> MRSKRFEALAKRPVNQDGFVKEWIEEGFIAMESPNDPKPSIKIVNGAVTELDGKPVSDFDLIDHFIARYGINLNRAEEVMAMDSVKLANMLCDPNVKRSEIVPLTTAMTPAKIVEVVSHMNVVEMMMAMQKMRARRTPSQQAHVTNVKDNPVQIAADAAEGAWRGFDEQETTVAVARYAPFNAIALLVGSQVGRPGVLTQCSLEEATELKLGMLGHTCYAETISVYGTEPVFTDGDDTPWSKGFLASSYASRGLKMRFTSG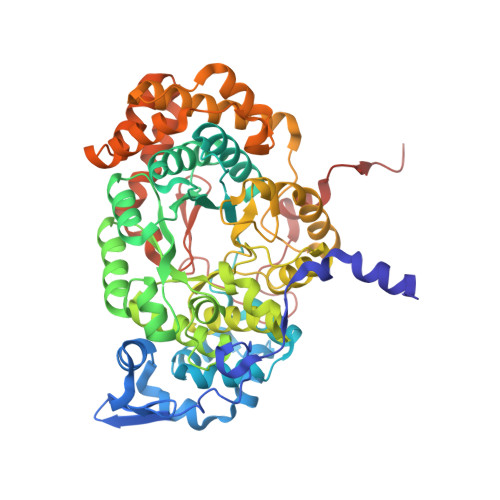SGSEVQMGYAEGKSMLYLEARCIYITKAAGVQGLQNGSVSCIGVPSAVPSGIRAVLAENLICSSLDLECASSNDQTFTHSDMRRTARLLMQFLPGTDFISSGYSAVPNYDNMFAGSNEDAEDFDDYNVIQRDLKVDGGLRPVREEDVIAIRNKAARALQAVFAGMGLPPITDEEVEAATYAHGSKDMPERNIVEDIKFAQEIINKNRNGLEVVKALAQGGFTDVAQDMLNIQKAKLTGDYLHTSAIIVGDGQVLSAVNDVNDYAGPATGYRLQGERWEEIKNIPGALDPNEID> GAALALLGDLVASVSEAAAATGFSVAEIAAGEAAAAIEVQIASLATVEGITSTSEAIAAIGLTPQTYAVIAGAPGAIAGFAALIQTVSGISSLAQVGYRFFSDWDHKVSTVGLYQQSGMALELFNPDEYYDILFPGVNTFVNNIQYLDP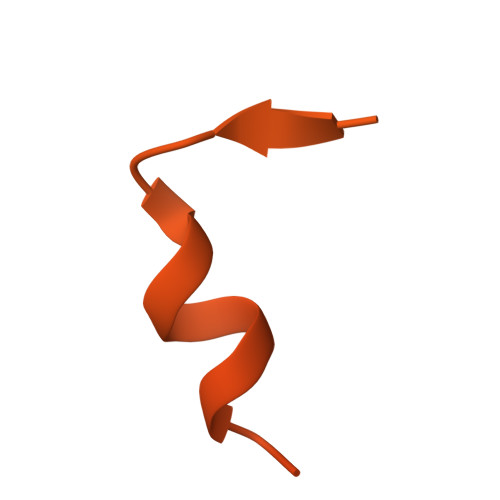RHWGPSLFATISQALWHVIRDDIPSITSQELQRRTERFFRDSLARFLEETTWTIVNAPINFYNYIQQYYSDLSPIRPSMVRQVAEREGTRVHFGHTYSIDDADSIEEVTQRMDLRNQQSVHSGEFIEKTIAPGGANQRTAPQWMLPLLLGLYGTVTPALEAYEDGPNQKKRRVSRGSSQKAKGTRASAKTTNKRRSRSSRS> MELKHSISDYTEAEFLQLVTTICNADTSSEEELVKLVTHFEEMTEHPSGSDLIYYPKEGDDDSPSGIVNTVKQWRAANGKSGFKQG;> MESKRNKPGKATGKGKPVGDKWLDDAGKDSGAPIPDRIAD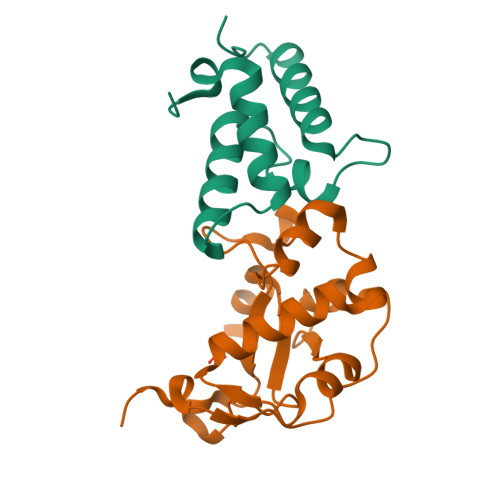KLRDKEFKSFDDFRKAVWEEVSKDPELSKNLNPSNKSSVSKGYSPFTPKNQQVGGRKVYELHHDKPISQGGEVYDMDNIRVTTPKRHIDIHRGK> MEPEDTQLKEDIKTTVNYIKQHGVEFENKLLEDERFSFIKKDDPLHEYYTKLMNEPTDTVSGEDNDRKSEREIARPPDFLFSQYDTGISRRDMEVIKLTARYYAKDKSIVEQMISKDGEARLNFMNSSHPLHKTFTDFVAQYKRVYSFTGQEIKKSKRTILDNCFERTQYWEFEKDKDREHDKLVE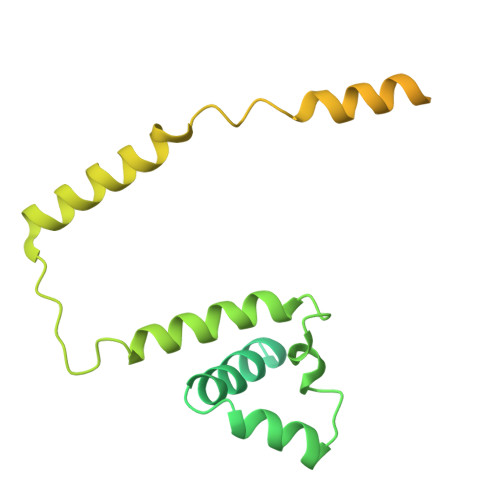LCKIQFAAIPWDKFTQVAKFSIPEDTEIFEGSLDLEQMRLRRVQTGIKLFDSIKPTNEEEKIVSDQGKQKGGDSKGKKRKIRAVGETRLKKSKK> KKIGLFYGTQTGKTESVAEIIRDEFGNDVVTLHDVSQAEVTDLNDYQYLIIGCPTWNIGELQSDWEGLYSELDDVDFNGKLVAYFGTGDQIGYADNFQDAIGILEEKISQRGGKTVGYWSTDG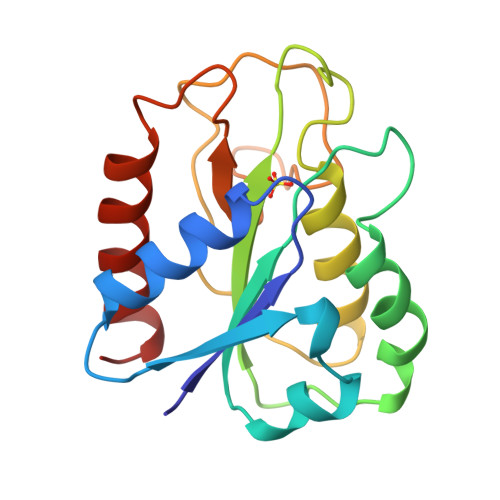YDFNDSKALRNGKFVGLALDEDNQSDLTDDRIKSWVAQLKSEFGL>[4x]AQESPAFIDPASWNTPFNGIAQVACHNCYEKQYANTFSSVLDSVRTLELDFWDQRDAVSGGSPHHWFVRHNPGTLFQSGNDNNCTGDGTGKNDLEACLNDVKNWSDKHPGHFPITLILDKKQGWSKESSGRTPKDFDELVARVFQGKLFTPQDLATHIGSGAGALQGNL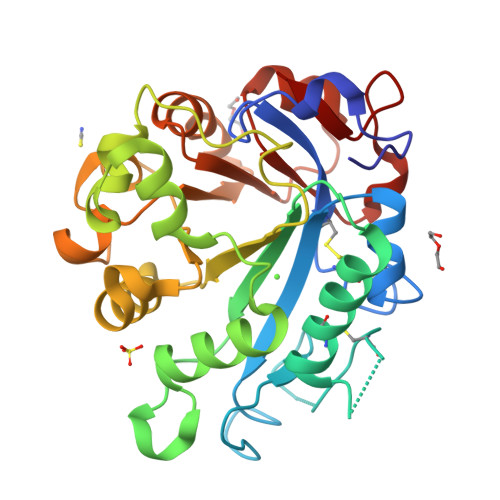KGKSWPTANDLQGKVLLVLNHSENQKLSQYAEARTSKAKVFISPVTNGQNDISGKVSGMSSQSSGYVAMNNMGKGDKSWAKQAFAYSHIGRVWGDDEVSFAQHINQKINLSAYYRFAAQSAGGYRIRPF> MGHIVANEKWRGSQLAQEMQGKIKLIFEDGLTPDFYLSNRCCILYVTEADLVAGNGYRKRLVRVRNSNNLKGIVVVEKTRMSEQYFPALQKFTVLDLGMVLLPVASQMEASCLVIQLVQEQTKEPSKNPLLGKKRALLLSEPSLLRTVQQ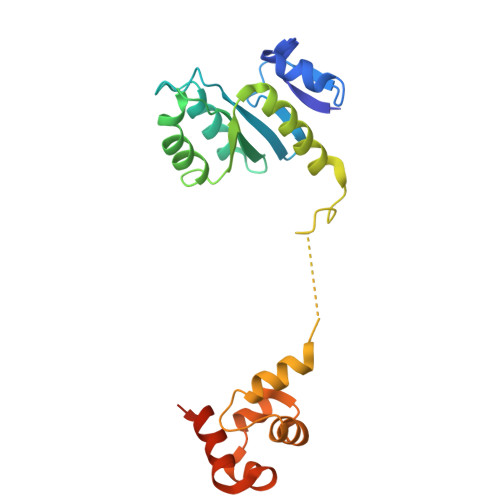IPGVGKVKAPLLLQKFPSIQQLSNASIGELEQVVGQAVAQQIHAFFTQPRLEHHHHHH NAD+-dependent protein deacylases (sirtuins) constitute a unique class of enzymes that are conserved from bacteria to humans. The human isotype Sirtuin 2 (Sirt2) deacetylates both nuclear and cytoplasmatic proteins and thereby functions as a major cell cycle regulator, a determinant of myelination, a regulator of autophagy and a suppressor of brain inflammation. In this work, we present the first crystal structures of Sirt2 in complex with a potent and Sirt2-selective small-molecule inhibitor with drug-like properties.

We solved the structure of Sirt2 in complex with SirReal2 and the cosubstrate NAD+ (structure termed Sirt2–SirReal2–NAD+) as well as in complex with SirReal2 and an acetyl-lysine peptide derived from histone H3 (residues 11–17, structure termed Sirt2–SirReal2-H3). Both Sirt2–SirReal2 crystals belonged to different monoclinic space groups and contained one monomer per asymmetric unit. Our structures feature a completely new and unexpected Sirt2 conformation, where SirReal2 functions as a ‘molecular wedge’ that traps Sirt2 in the open conformation even in the presence of an acetyl-lysine peptide substrate. We call this a ‘locked open’ state. The position of SirReal2 in the EC-site of Sirt2 is very similar in both structures with either NAD+ or the acetyl-lysine peptide substrate (r.m.s.d. of 0.47 Å), and we will primarily describe the binding of SirReal2 in the presence of NAD+, as this structure likely represents the SirReal2-inhibited form of the enzyme. Structural comparison of the available Sirt2 structures with the Sirt2–SirReal2–H3 complex can be found in Supplementary Fig. 3. In particular, the side chains of Phe235 and Tyr104 that usually cap the acetyl-lysine are rotated towards the surface of Sirt2. Surprisingly, this rearrangement does not prevent Sirt2 from binding its acetyl-lysine peptide substrate, but deacetylation and the domain closure is blocked effectively. The hydrophobic acetyl-lysine–binding tunnel is not formed in all Sirt2–SirReal structures, since Phe235, which usually caps the acetyl-lysine, is rotated ~90° towards the surface. Further thermal stability experiments indicated an additional stabilization of the Sirt2–SirReal2 complex in the presence of either NAD+ or a peptidic acetyl-lysine substrate. These findings were the key to a successful crystallization of Sirt2 in complex with SirReal2 that was only achieved in the presence of either substrate or cosubstrate.

> GHMERLLDELTLEGVARYMQSERCRRVICLVGAGISTSAGIPDFRSPSTGLYDNLEKYHLPYPEAIFEISYFKKHPEPFFALAKELYPGQFKPTICHYFMRLLKDKGLLLRCYTQNIDTLERIAGLEQEDLVEAHGTFYTSHCVSASCRHEYPLSWMKEKIFSEVTPKCEDCQSLVKPDIVFFGESLPARFFSCMQSDFLKVDLLLVMGTSLQVQPFASLISKAPLSTPRLLINKEKAGQSDPFLGMIMGLGGGMDFDSKKAYRDVAWLGECDQGCLALAELLGWKKELEDLVRREHASIDAQS;> TGGKAPR> GMGRIEVVNVSHIFHRGTPLEKKALENVSLVINEGECLLVAGNTGSGKSTLLQIVAGLIEPTSGDVLYDG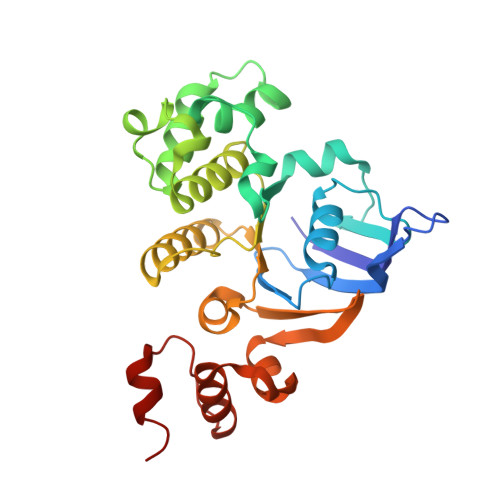ERKKGYEIRRNIGIAFQYPEDQFFAERVFDEVAFAVKNFYPDRDPVPLVKKAMEFVGLDFDSFKDRVPFFLSGGEKRRVAIASVIVHEPDILILDEPLVGLDREGKTDLLRIVEKWKTLGKTVILISHDIETVINHVDRVVVLEKGKKVFDGTRMEFLEKYDPRFFTSKMLVMRRLVLKGEDPFSMSDDELLERVCNS> SMFYGTVSSPDSGVYEMKIGSIIFQVASGDITKEEADVIVNSTSNSFNLKAGVSKAILECAGQNVERECSQQAQQRKNDYIITGGGFLRCKNI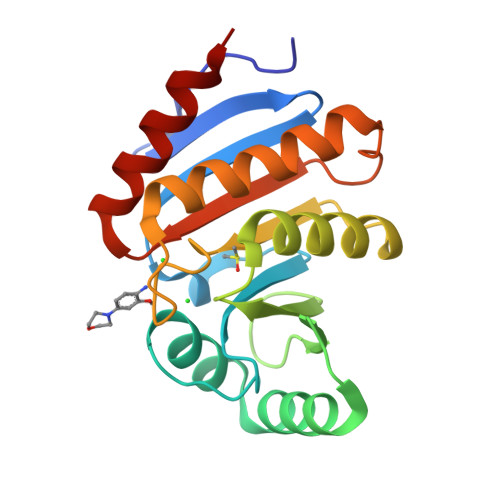IHVIGGNDVKSSVSSVLQECEKKNYSSICLPAIGTGNAKQHPDKVAEAIIDAIEDFVQKGSAQSVKKVKVVIFLPQVLDVFYANMKKREG>HAALRFKHPVDRVAPTTQTPQIQLQPSSPGSTKTCQADPYIMPPLPFTEWLPRKNYTRAYFRPRFVSPRAEFSSLEDINVPVLPPMTVLERGMVVSPDNKDPSLPCPPIIDVDVAADDAVDETEKLLFGLATTADRLDRLLPSLLYSYGNTKAGIIVLVPESDDDLDKQMTYFRNRGLDLTLIKSPLDFTARYFGLVQAFAEHIRTKRPQTTWVSFIDDDTFWLSLPTVAEELKLFDVNKKHYIGALSEASWQVDTFGHIAFGGAGVFVSKPLLDVLEQYYDECQSWGEQPGDQKLGQCIQKYGDTPLTLWPSLYQMDMKGEVDGVYESGRKIESLHHWNSWYTKDVVKMTTVAAAAGRKSVLRRWVFDQEEYVNNSTGKSVRTFWVMTNGYSLVKYTYDENTPDDAINFDHTEKTWEEDPRGYEGRLGPLRLKDQAGVTKDRWLLREAYVVGDNVHQWYVREEDEGHSVIEIVWLGPKGGGGAGVHDYAVRKQH[2x]

UDP-α-D-galactofuranose (UDP-Galf): β-galactofuranoside β-(1→5)-galactofuranosyltransferase, known as GfsA, is essential in synthesizing β-(1→5)-galactofuranosyl oligosaccharides that are incorporated into the cell wall of pathogenic fungi. GfsA is an enzyme that transfers β-galactofuranose from UDP-α-D-galactofuranose to the 5ʹ-OH of β-galactofuranose. In addition to the typical GT-A fold domain, GfsA has a unique domain formed by the N and C termini. GfsA functions as an inverting enzyme, catalyzing the transfer of a Galf residue from UDP-α-Galf to the 5ʹ-OH of a β-galactofuranoside substrate, leading to the formation of a Galf-β-(1→5)-Galf product.

In this study, we present the crystal structure of GfsA-Mn2+-UDP and Galf, the β-Galf β-(1→5)-galactofuranosyltransferase from A. fumigatus. A diffraction dataset with a resolution of 2.46–2.37 Å was obtained for a crystal of GfsA–Mn2+–UDP and Galf complex. Para-nitrophenyl (pNP)-β-Galf was used in crystallization; however, the pNP group's electron density was unresolved. The complex of GfsA–Mn2+–UDP and Galf is dimeric, aligning well with the gel filtration chromatography findings. There were a domain with a GT-A fold domain (α-helical domain) that includes the central region (spanning residues 160–360) and a GfsA-specific domain (β-sandwich domain) that includes the N- and C-terminal regions (residues 76–159 and 361–535). The UDP, a product of the donor substrate, was coordinated with Mn2+ through interactions with the DXD motif (D260, D262, and H379). UDP interacted with W384, H380, and S383 regarding the phosphate group, while A173, R178, F231, I259, and D261 interacted with the uracil moiety. The acceptor substrate, Galf, was present within the depression and hydrogen bonded with D335 and D360. D360 precisely orients the acceptor substrate by forming a hydrogen bond with the 3ʹ-OH group of the acceptor Galf. In our study, the crystal structure revealed that the β-galactofuranoside had its 1ʹ-OH group oriented outward from the active site.>[8x]MAAKRYTSMAYANADEMTFGVSKYPVKAGLDLEIGAGYTIPEINYAPRPEAGASKEKLIKEYERITTDVMERMVQVGFPAIILETEHVQQMSNNPSWGAEVAHAQKTIMEKYHDEYGIKCALRHTIGDIRENREFLQLRGDKYSVFLEAFEQCAENGADLLSVESMGGKEVFDYAVLRNDIPGLLYSIGCLGSIDMELIWTDISKIAKKTGTISAGDTDCAQANTAMFIGGGLLNKNLAHTIAVIARAISAPRSLVAYEAGAVGPGKDCGYENIIVKAITGMPMTMEGKTSTCAHSDVMGNLVMQCCDCWSNESVEYHGEFGGTTVQCWSETLAYDCALMNTALETKNDKVLRDLMMLSDRYRDPQAYMLAYDNAYRVGQSIVKDGDNIYLRAKNAAIECCNIIEEGAAGKLELSRF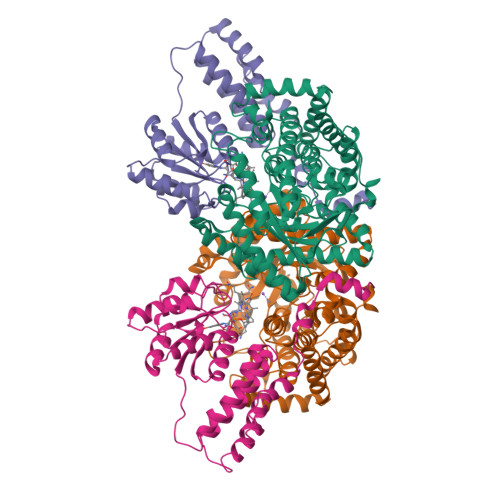ETKALADAKAALEALPDDMDKFMDDCLTKYKSEVKVFKPENYGF;>[8x]MLDFTEASLKKVLTRYNVALEKALTPEEAAEELYPKDELIYPIAKAIFEGEEDDVVEGLQAAIEAGKDPIDLIDDALMVGMGVVIRLYDEGVIFLPNVMMSADAMLEGIEYCKENSGATPKTKGTVVCHVAEGDVHDIGKNIVTALLRANGYNVVDLGRDVPAEEVLAAVQKEKPIMLTGTALMTTTMYAFKEVNDMLLENGIKIPFACGGGAVNQDFVSQFALGVYGEEAADAPKIADAIIAGTTDVTELREKFHKH> MAHHHHHHGHHHQLENLYFQGEETAVPENSGANTELVSGESEHSTNEADKQNEGEHARENKLEKAEGVATASETASPASNEAATTETAEAASAAKPEEKASEVVAETPSAEAKPKSDKETEAKPEATNQGDESKPAAEANKTEKEVQPDVPKNTEKTLKPKEIKFNSWEELLKWEPGAREDDAINRGSVVLASRRTGHLVNEKASKEAKVQALSNTNSKAKDHASVGGEEFKAYAFDYWQYLDSMVFWEGLVPTPDVIDAGHRNGVPVYGTLFFNWSNSIADQERFAEALKQDADGSFPIARKLVDMAKYYGYDGYFINQETTGDLVKPLGEKMRQFMLYSKEYAAKVNHPIKYSWYDAMTYNYGRYHQDGLGEYNYQFMQPEGDKVPADNFFANFNWDKAKNDYTIATANWIGRNPYDVFAGLELQQGGSYKTKVKWNDILDENGKLRLSLGLFAPDTITSLGKTGEDYHKNEDIFFTGYQGDPTGQKPGDKDWYGIANLVADRTPAVGNTFTTSFNTGHGKKWFVDGKVSKDSEWNYRSVSGVLPTWRWWQTSTGEKLRAEYDFTDAYNGGNSLKFSGDVAGKTDQDVRLYSTKLEVTEKTKLRVAHKGGKGSKV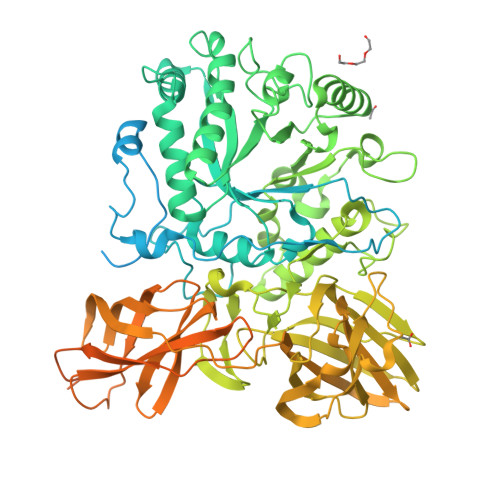YMAFSTTPDYKFDDADAWKELTLSDNWTNEEFDLSSLAGKTIYAVKLFFEHEGAVKDYQFNLGQLTISDNHQEPQSPTSFSVVKQSLKNAQEAEAVVQFKGNKDADFYEVYEKDGDSWKLLTGSSSTTIYLPKVSRSASAQGTTQELKVVAVGKNGVRSEAATTTFDWGMTVKDTSLPKPLAENIVPGATVIDSTFPKTEGGEGIEGMLNGTITSLSDKWSSAQLSGSVDIRLTKSRTVVRWVMDHAGAGGESVNDGLMNTKDFDLYYKDADGEWKLAKEVRGNKAHVTDITLDKPITAQDWRLNVVTSDNGTPWKAIRI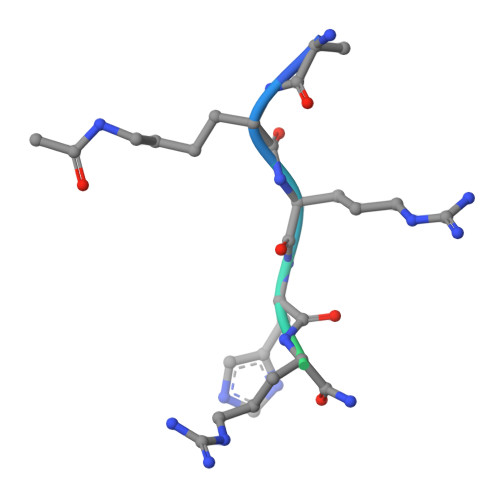> AKRHRKILRNSIQGI> SRVFLDHNALPDTLKVTYDSFCSNGVTHRNQPRGDCDGVQINVPITFQVKVTATECIQEQSFVIRALGFTDIVTVQVLPQCECRCRDQSRDRSLCHGKGFLECGIC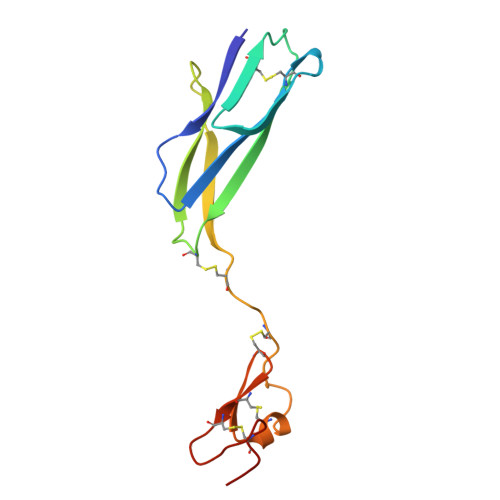RCDTGYIGKNCEHH>SHMERVFVWDLDETIIIFHSLLTGTFASRYGKDTTTSVRIGLMMEEMIFNLADTHLFFNDLEDCDQIHVDDVSSDDNGQDLSTYNFSADGFHSSAPAANLCLGSGVHGGVDWMRKLAFRYRRVKEMYNTYKNNVGGLIGTPKRETWLQLRAELEALTDLWLTHSLKALNLINSRPNCVNVLVTTTQLIPALAKVLLYGLGSVFPIENIYSATKTGKESCFERIMQRFGRKAVYVVIGDGVEEEQGAKKHNMPFWRI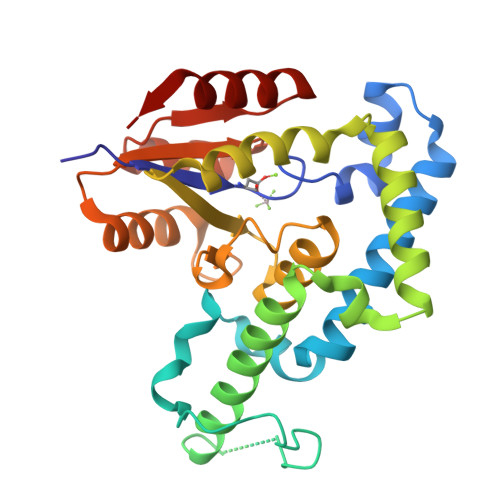SCHADLEALRHALELEYL[4x]> GEVNKIIGSRTAGEGAMEYLIEWKDGHSPSWVPSSYIAADVVSEYETPW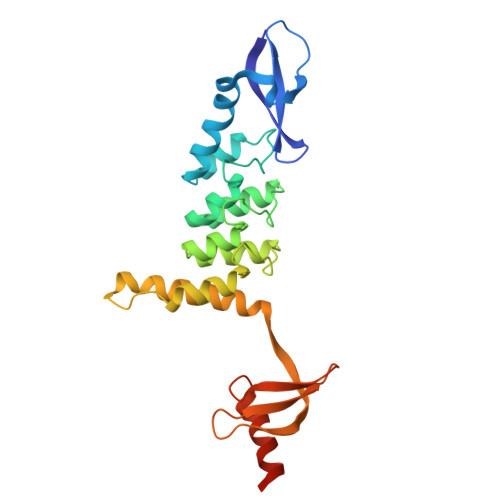WTAARKADEQALSQLLEDRDVDAVDENGRTALLFVAGLGSDKCVRLLAEAGADLDHRDMRGGLTALHMAAGYVRPEVVEALVELGADIEVEDERGLTALELAREILKTTPKGNPMQFGRRIGLEKVINVLEGQVFEYAEVDEIVEKRGKGKDVEYLVRWKDGGDCEWVKGVHVAEDVAKDYEDGLEYAVAESVIG>[2x]MCP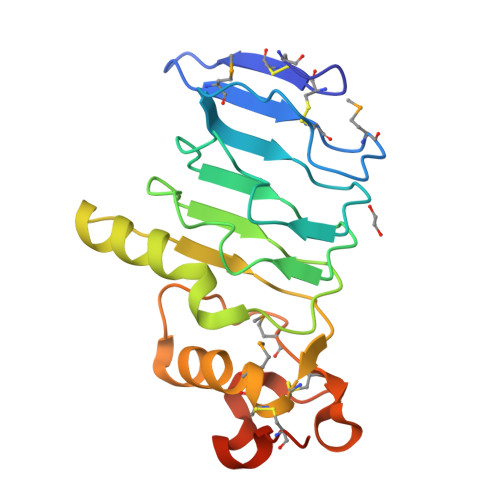SACKCTVSLYGEMVVACGGMGLTEIPEDIPHRAVYLVLKDNNITKITSYSFKGLRNLQGIDLSNNKINHISSAALRHLGHLDDIDLSRNELTSVSEKLFDFPISSAKAQGRRFFVYLANNPWGCDCRMAWLAQELAGGSKTFGDRHMECATPAALAGRGLSEIPQTSFVCTGRDISFDSD>MTTVTSYPGVYIEELNSLALSVSNSATAVPVFAVDEQNQYISEDNAIRINSWMDYLNLIGNFNNEDKLDVSVRAYFANGGGYCYLVKTTSLEKIIPTLDDVTLLVAAGEDIKTTVDVLCQPGKGLFAVFDGPETELTINGAEEAKQAYTATPFAAVYYPWLKADWANIDIPPSAVMAGVYASVDLSRGVWKAPANVALKGGLEPKFLVTDELQGEYNTGRAINMIRNFSNTGTTVWGARTLEDKDNWRYVPVRRLFNSVERDIKRAMSFAMFEPNNQPTWERVRAAISNYLYSLWQQGGLAGSKEEDAYFVQ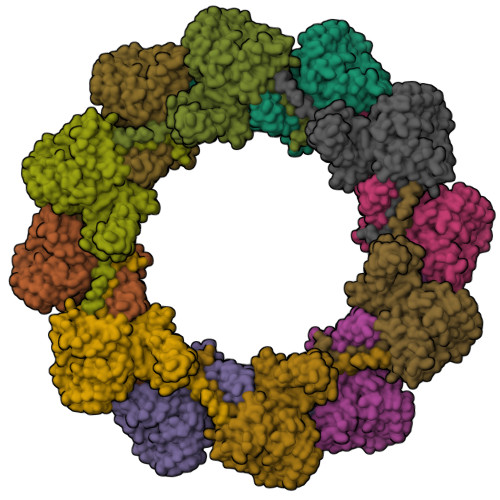IGKGITMTQEQIDAGQMIVKVGLAAVRPAEFIILQFTQDVEQR[12x]>[4x]MERQVLLSEPEEAAALYRGLSRQPALSAACLGPEVTTQYGGRYRTVHTEWTQRDLERMENIRFCRQYLVFHDGDSVVFAGPAGNSVETRGELLSRESPSGTMKAVLRKAGGTGTAEEKQFLEVWEKNRKLKSFNLSALEKHGPVYEDDCFGCLSWSHSETHLLYVADKKRPKAESFFQTKALDVTGSDDEMARTKKPDQAIKGDQFLFYEDWGENMVSKSTPVLCVLDIESGNISVLEGVPESVSPGQAFWAPGDTGVVFVGWWHEPFRLGIRFCTNRRSALYYVDLTGGKCELLSDESVAVTSPRLSPDQCRIVYLRFPSLVPHQQCGQLCLYDWYTRVTSVVVDIVPRQLGEDFSGIYCSLLPLGCWSADSQRVVFDSPQRSRQDLFAVDTQMGSVTSLTAGGSGGSWKLLTIDRDLMVVQFSTPSVPPSLKVGFLPPAGKEQAVSWVSLEEAEPFPDISWSIRVLQPPPQQEHVQYAGLDFEAILLQPSNSPEKTQVPMVVMPHGGPHSSFVTAWMLFPAMLCKMGFAVLLVNYRGSTGFGQDSILSLPGNVGHQDVKDVQFAVEQVLQEEHFDAGRVALMGGSHGGFLSCHLIGQYPETYSACVVRNPVINIASMMGSTDIPDWCMVEAGFSYSSDCLPDLSVWAAMLDKSPIKYAPQVKTPLLLMLGQEDRRVPFKQGMEYYRVLKARNVPVRLLLYPKSTHALSEVEVESDSFMNAVLWLCTHLGS

Acylpeptide hydrolase (APEH) or acylaminoacyl‐peptidase (AAP) is a serine hydrolase that regulates protein metabolism. It can also bind to and process unusual substrates, acting as a detoxifier. The most prominent physiological function of APEH is the removal of N‐acetylated amino acids from the N‐terminus of oligopeptides and proteins (Perrier et al., 2005) thereby exerting crucial control over the proteasomal degradation of damaged and misfolded proteins (Adibekian et al., 2011; Hoernstein et al., 2023; Hwang et al., 2010; Palmieri et al., 2011; Sandomenico et al., 2021; Shimizu et al., 2003; Shimizu et al., 2004; Tangri et al., 2021). The S9 serine protease subfamily, the so‐called oligopeptidases, employs a further, size‐based selection process (Kobayashi & Smith, 1987). Their active site is sequestered in an inner pocket that is formed between the catalytic hydrolase domain and a propeller domain that caps it.

The pAPEH—dimethoxy‐phosphate (DMP) complex was created by adding dichlorvos (DDVP), an organophosphate insecticide, to pAPEH. The structure of the complex was determined by cryo‐EM to 2.65 Å maximal resolution, in D2 symmetry. Dimethoxy‐phosphate (DMP) residue of dichlorvos is bound covalently to the active Ser587 (Oγ‐P1) of APEH. The free oxygen of the phosphate (P1‐O1 moiety) is fixed and oriented by the oxyanion site. Here—in contrast to the pAPEH‐AcAMHK complex—one H‐bond is actually formed with the oxyanion‐loop (with the amide NH of Gly509), while the other interaction partner (the amide NH of His588) is still too far for a strong association. One of the methoxy groups is positioned within the S1 binding pocket. Compared to ligand‐free pAPEH, the shift of the oxyanion‐ and the His‐loops can be seen: the oxyanion‐loop moves closer to the inhibitor with the backbone N and Cα of Gly509 shifting by 0.6 and 0.7 Å, respectively, in similar way to that seen in the pAPEH‐AcAMHK complex, however, the catalytic His‐loop moved in the opposite direction (by 0.8 Å measured between His707(Cα)s), shifting away from the catalytic center. We found DMP bound in a non‐aged form—meaning that it retains both of its methoxy substituents. Aging is the spontaneous dealkylation process that often occurs in organophosphates bound to serine proteases, where the gradual loss of the O‐alkyl (or N‐alkyl) groups increases the irreversibly bound nature of the complex. On the other hand, surprisingly, through this very same sensitivity toward the OPs, APEH has also become a potential target for cognitive enhancing drugs promoting synaptic plasticity and learning in young brains (García‐Rojo et al., 2017; Sandoval et al., 2012). Both developing sensitive and specific monitoring systems and attempting to design nontoxic but effective inhibitors of APEH require a precise understanding of the mode and requirements of the binding process—the structure of the pAPEH‐OP complex presented here can be utilized toward these goals.To further explore this issue, we have conducted biochemical and crystallographic studies on the interactions of six GSTOs from T. versicolor with chemical libraries. The six TvGSTOs (named TvGSTO1S to TvGSTO6S) used in this study are representatives of the twelve TvGSTOs that have a catalytic serine, while four others have a cysteine instead. In this study, we demonstrated at the biochemical and structural level that T. versicolor GSTs that belong to the Omega class interact with polyphenolic compounds found in wood, and in particular with flavonoids such as dihydrowogonin and naringenin. The ability of TvGSTOs to bind polyphenols through different sites suggests that fungal GSTs could be involved in the transport of various polyphenols.

The structure of apo TvGSTO3S was determined by X-ray crystallography at a resolution of 1.35 Å. It has a typical GST fold where the N-terminal thioredoxin domain of one monomer cross-interacts with the C-terminal all-helical domain of the second one, and vice-versa. TvGSTO3S displays the highest sequence identity with Omega GSTs, though its closest structural homologs identified by PDBeFold23 are Tau GSTs. The N-terminal end of TvGSTO3S helix α1 harbors a serine as the catalytic residue instead of the cysteine found in the other GSTOs structurally characterized so far17,25. It enables efficient GSH-transferase activity towards usual synthetic substrates and disables reductase activity.

>[2x]MSSTKQITLYTATFSPYAHRVRIALEEAGAEYTTYDVDILRNMPDWFPLVNPLKKIPAMTFGGPEVPPDQPSPESAKIAESLAMLEFIADLFPDAKLLPTDPVLRARARTFMALYENYVNGQFRDVWFLGTPADPLLQALEMLQGALPPDGGFAAGEWSIADAAVIPFLARMFPYLEAGLGLYSKEDGVKMRKAMASERFARIRQYVRDCRARPSFANTWAGDAEQVEAAKTVPMLRVGEHHHHHH GDF-5, like BMP-2 and BMP-4, binds to and oligomerizes two types of serine-/threonine kinase transmembrane receptors, termed TGF-β superfamily type I and type II receptors. Whereas BMP-2 binds to both type I receptors—BMPR-IA and BMPR-IB—with similar affinities, GDF-5 exhibits a 12-fold higher affinity for BMPR-IB than for BMPR-IA. This type I receptor specificity of GDF-5 is due to a single amino acid, Arg57, which is located in the pre-helix loop of the ligand. Mutation of Arg57 in GDF-5 to alanine abrogates type I receptor specificity completely, whereas the mutation of Arg57 to leucine leads to enhanced binding to BMPR-IA and attenuated type I receptor specificity.

Structural studies were performed by crystallizing the binary complex of GDF-5 R57A bound to BMPR-IA and determining its structure at high resolution. Although a full complex—one GDF-5 R57A dimer and two BMPR-IAEC molecules —was observed in the asymmetric unit of the crystal, the backbone of the ligand–receptor complex was highly symmetrical, as shown from the superposition of the two GDF-5 monomers as well as the BMPR-IA ectodomains. Analysis of the two binding interfaces formed by the homodimeric GDF-5 and the two BMPR-IA molecules yielded a total of 18 intermolecular hydrogen bonds (H-bonds), suggesting that polar bonds play a role in GDF-5 type I receptor recognition and binding. Upon binding of GDF-5 R57A to BMPR-IAEC, the backbone atoms of residues Phe97 to Val104 (finger 2) and Lys29 to Ile38 (ω-loop in finger 1) of GDF-5 R57A moved up by 5.5 Å towards BMPR-IA, although residues in the very tips of finger 2 shared no contact with BMPR-IA. With regards side chain rearrangements, the largest changes were observed for the two tryptophans in the wrist epitope of GDF-5 R57A; Trp33 moved downwards by about 4 Å and Trp36 rotated from a highly solvent-exposed conformation into a position located above Trp33 thereby moving by almost 10 Å. In complex with GDF-5 R57A, the α-helix of BMPR-IA formed similarly as seen in the complex with BMP-2, consistent with the observation in the study of Klages et al. that small changes in the environment result in spontaneous α-helix formation. Although the structures of the ligands as well as of BMPR-IA were almost identical in the different complexes with varying binding partners, superposition of the complexes of GDF-5 R57A:BMPR-IA and BMP-2:BMPR-IA revealed that the orientation/position of the receptor ectodomain in its binding site differed between these complexes. From this comparison we determined that the membrane-distal part of the BMPR-IA molecules swiveled towards the N-terminal end of the GDF-5 R57A α-helix and further into the concave wrist epitope, whereas the membrane-proximal half of the receptor swung out of the binding site compared to the receptor orientation observed for the BMP-2:BMPR-IA complex.

>MKRQGKRPSKNLKARCSRKALHVNFKDMGWDDWIIAPLEYEAFHCEGLCEFPLASHLEPTNHAVIQTLMNSMDPESTPPTCCVPTRLSPISILFIDSANNVVYKQYEDMVVESCGCR[2x];>[2x]GSGAMAQNLDSMLHGTGMKSDSDQKKSENGVTLAPEDTLPFLKCYCSGHCPDDAINNTCITNGHCFAIIEEDDQGETTLASGCMKYEGSDFQCKDSPKAQLRRTIECCRTNLCNQYLQPTLPPVVIGPFFDGSIR>[2x]MDLTVEPNLHSLITSTTHKWIFVGGKGGVGKTTSSCSIAIQMALSQPNKQFLLISTDPAHNLSDAFGEKFGKDARKVTGMNNLSCMEIDPSAALKDMNDMAVSRANNNGSDGQGDDLGSLLQGGALADLTGSIPGIDEALSFMEVMKHIKRQEQGEGETFDTVIFDTAPTGHTLRFLQLPNTLSKLLEKFGEITNKLGPMLNSFMGAGNVDISGKLNELKANVETIRQQFTDPDLTTFVCVCISEF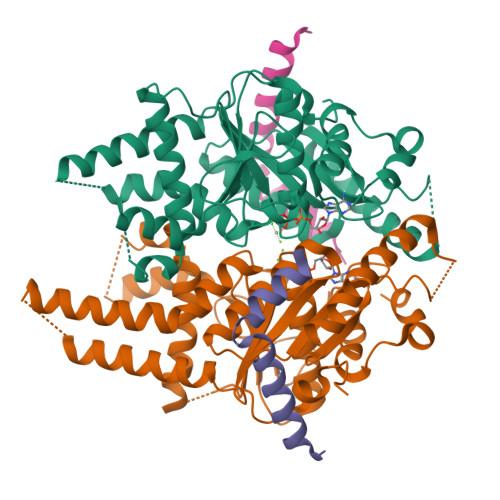LSLYETERLIQELISYDMDVNSIIVNQLLFAENDQEHNCKRCQARWKMQKKYLDQIDELYEDFHVVKMPLCAGEIRGLNNLTKFSQFLNKEYNPITDGKVIYELEDKE;>MSELTEAEKRRLLRERRQKKFSNGGASSRLNKITGQAS[2x]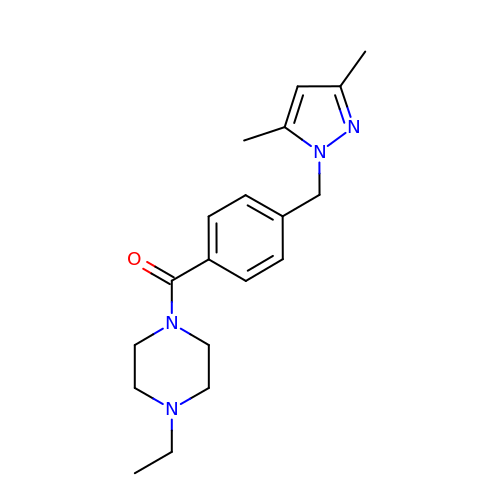{4-[(3,5-dimethyl-1H-pyrazol-1-yl)methyl]phenyl}(4-ethylpiperazin-1-yl)methanone | C19 H26 N4 O | XFIDMUXINICVOV-UHFFFAOYSA-N1-[(3S)-1-{[3-(3-chlorophenoxy)-4-hydroxyphenyl]sulfonyl}piperidin-3-yl]-5-methylpyrimidine-2,4(1H,3H)-dione 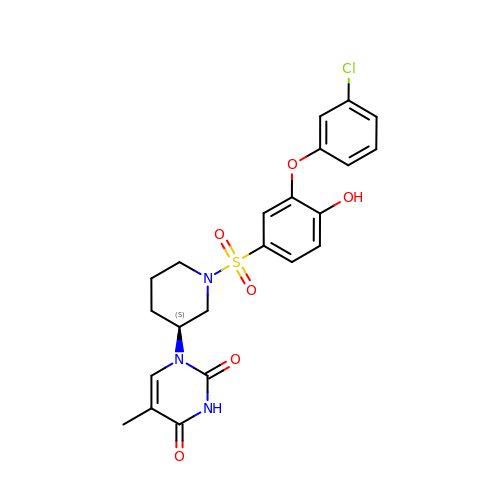| C22 H22 Cl N3 O6 S | IDMZBDJWQBWWLK-INIZCTEOSA-N>[2x]ILPDSVDWREKGCVTEVKYQGSCGACWAFSAVGALEAQLKLKTGKLVSLSAQNLVDCSTEKY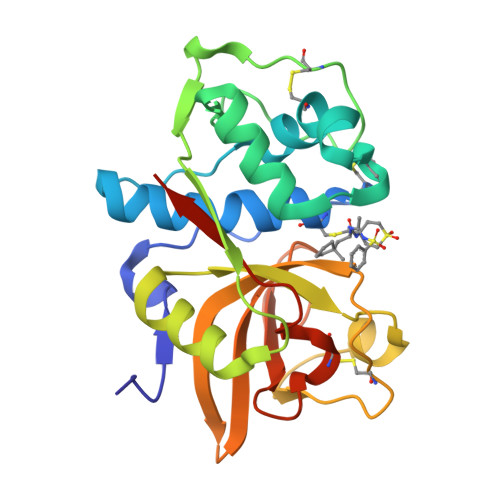GNKGCNGGFMTTAFQYIIDNKGIDSDASYPYKAMDQKCQYDSKYRAATCSKYTELPYGREDVLKEAVANKGPVSVGVDARHPSFFLYRSGVYYEPSCTQNVNHGVLVVGYGDLNGKEYWLVKNSWGHNFGEEGYIRMARNKGNHCGIASFPSYPEIGHHHHHH We identified DR1245, a protein of unknown function conserved only in the Deinococcaceae, as a DdrB partner in cells recovering from ionizing radiation treatment. Our study indicates that cells devoid of DR1245 grow more slowly under normal (unstressed) growth conditions than wild-type cells, but are as radioresistant as wild type. The three-dimensional structure of DR1245 revealed its strong structural homology with type III secretion system (T3SS) chaperones and with the YbjN homolog from Synechococcus elongatus. Thus, the DR1245 protein might have some chaperone activity towards DdrB and possibly other substrates.

To determine the phases, native DR1245 were formed in the presence of potassium bromide and 2 Å resolution electron density maps were produced by single-wavelength anomalous dispersion and a molecular model was built. The asymmetric unit was composed of two monomers, which corroborates the results from the size exclusion chromatography presented above. The final model includes 301 of the 306 residues from the dimer, including residues 2 to 153, and 4 to 152, of monomers A and B, respectively. Each DR1245 monomer comprises 3 α-helices packed against one side of a twisted six-stranded anti-parallel β-sheet with an α-β-β-β-α-β-β-α topology. The DR1245 dimerization interface involves residues from the β3 to β4 loop that interact with the beginning of the α3 helix of the other monomer. The surface area buried per monomer in the dimer interface is 1,425 Å2 or 15.4% of the total surface area, as defined by the PISA server. Interestingly, the dimerization interface harbors a cavity that contains water molecules and the bromide ion. A sulfate and a potassium ion are localized at both sides of the cavity and are each coordinated by the His129 from one monomer and Arg59 from the other monomer. The two monomers are highly symmetrical except for their unstructured 11 C-terminus residues. The C-terminus from monomer A is packed against its α3 helix and β2 strand whereas the C-terminus from monomer B protrudes away to interact with the C-terminus of the A monomer from a symmetric neighboring molecule.

>[2x]METALLTLDTLAKYLQEKEVQLDIEENGGQRFIRMGWRFEMGDAAVLVSVNDGPNNTSRLEITCVTQKTYADRRAEVAMMLNDRNRERAFARSIDQEGNVWLEYVGFYPTLAEMPQETFDTLFGGVLMHFQDDYAALEGYVPQEGMQIQQPQA>MVQVLSVLVIPLLTLF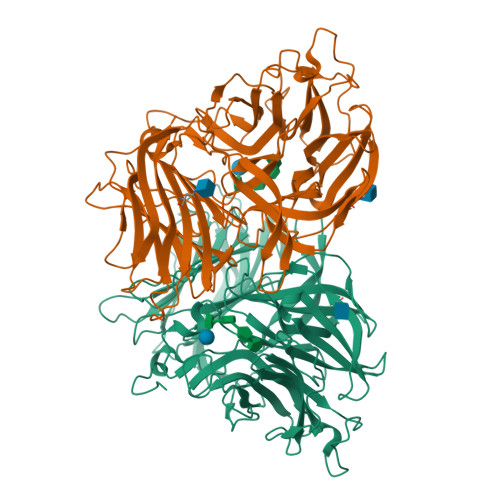FGYVASSSIDLSVDTSEYNRPLIHFTPEKGWMNDPNGLFYDKTAKLWHLYFQYNPNATAWGQPLYWGHATSNDLVHWDEHEIAIGPEHDNEGIFSGSIVVDHNNTSGFFNSSIDPNQRIVAIYTNNIPDNQTQDIAFSLDGGYTFTKYENNPVIDVSSNQFRDPKVFWHEDSNQWIMVVSKSQEYKIQIFGSANLKNWVLNSNFSSGYYGNQYACPGLIEVPIENSDKSKWVMFLAINPGSPLGGSINQYFVGDFDGFQFVPDDSQTRFVDIGKDFYAFQTFSEVEHGVLGLAWASNWQYADQVPTNPWRSSTSLARNYTLRYVHTNAETKQLTLIQNPVLPDSINVVDKLKKKNVKLTNKKPIKTNFKGSTGLFDFNITFKVLNLNVSPGKTHFDILINSQELNSSVDSIKIGFDSSQSSFYIDRHIPNVEFPRKQFFTDKLAAYLEPLDYDQDLRVFSLYGIVDKNIIELYFNDGTVAMTNTFFMGEGKYPHDIQIVTDTEEPLFELESVIIRELNK[4x]>[2x]QNVGTQAAEEPLNLPISVCTAPGNCQTEADAVVLDSNWRWAHTTTGYTNCYTGNLWDTTLCPTPETCTTNCAIDGVPLADWSGTYGGSVTGNKFNLKFVTVGPYSTNIGARTFLLDSTKTRYRMFQLLNREFTYDVDVSSLDCGLNGALYFVSMDADGGAAKYPTNKGGAKYGTGYCDAQCPHDVKWINGLANSKDWTPIPGDANSGKGYYGNCCAELDIWEANKQSQAFTTHPCTPNDQTRCEGVVCGDNDSGDRYNGMCDKDGCDFASYRMNDHTFYGPGSTFKLDSTKPFTVVSQFITTDGTDNGDFKEFRRFYVQNGVRIENSKVNFPGITAYDSITDEMCAATKGLFGDLDDHKNKGGMKQMGEAMRKGMALVMSIWDDHDVNMLWLDSNYPPTGNPSTPGVARGPCPTTSGVPSEVEVTQANAVVSFGNIKFGPIGSTV

During macromolecular X-ray crystallography experiments, protein crystals held at 100 K have been widely reported to exhibit reproducible bond scission events at doses on the order of several MGy. OH-cleavage from tyrosine residues is regularly cited as amongst the most available damage pathways in protein crystals at 100 K, despite a lack of widespread reports of this phenomenon in protein crystal radiation damage studies. A systematic investigation performed on a range of protein crystal damage series deposited in the Protein Data Bank has established that Tyr –OH electron density loss is not generally a dominant damage pathway in protein crystals at 100 K. Full Tyr aromatic ring displacement is here proposed to account for instances of observable Tyr –OH electron density loss, with the original myrosinase data shown to be consistent with such a damage model. To better characterize the reproducibility of Tyr –OH group electron density loss in irradiated protein crystals, we have performed a systematic investigation on a wide range of structures at 100 K. A subset of previously conducted MX radiation damage investigations have included deposition of readily accessible coordinate and structure factor information in the Protein Data Bank (PDB), providing an ideal database of protein damage series.

Regardless of the feasibility of a radiation-induced Tyr –OH damage event within crystalline protein at 100 K, Tyr –OH density loss is in general significantly lower than for Glu and Asp carboxyl­ates for doses >1 MGy, at which de­carboxyl­ation events were reported. Prominent Tyr –OH density loss did not appear to be a widespread feature of general protein structures, a finding that is consistent with the high energetic barrier for Tyr phenolic C—O bond scission.(S,S)-(-)-N,N'-DI-5'-[5',6',7',8'-TETRAHYDRO- 2'(1'H)-QUINOLYNYL]-1,10-DIAMINODECANE 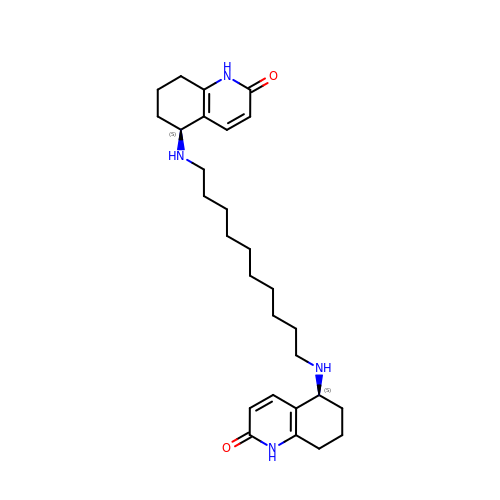DIHYDROCHLORIDE | C28 H42 N4 O2 | CKFAWHBPSZAYLS-ZEQRLZLVSA-N>ADSDVPNDILEEQLYNSIVVADYDSAVEKSKHLYEEKKSEVITNVVNKLIRNNKMNCMEYAYQLWLQGSKDIVRDCFPVEFRLIFAENAIKLMYKRDGLALTLSNDVHGNDGRLAFGDGKDKTSPKVSWKFIALWENNKVYFKILNTERNQYLVLGVGTNPNGDHMAFGVNSVDSFRAQWY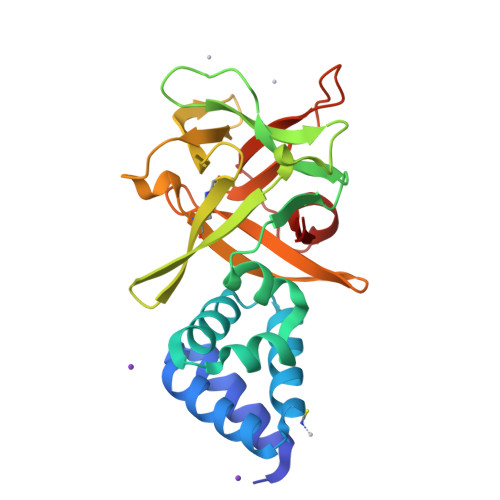LQPAKYDKDNLFYIYNREYSKALTLSRTLETSGNRMAWGYNGRVIGSPEHYAWGVKAF[2x]>MSRVPSPPPPAEMSSGPVAESWCYTQIKVVKFSYMWTINNFSFCREEMGEVIKSSTFSSGANDKLKWCLRVNPKGLDEESKDYLSLYLLLVSCPKSEVRAKFKFSILNAKGEETKAMESQRAYRFVQGKDWGFKKFIRRDFLLDEANGLLPDDKLTLFCEVSVVQDSVNISGQNTMNMVKVPECRLADELGGLWENSRFTDCCLCVAGQEFQAHKAILAARSPVFSAMFEHEMEESKKNRVEINDVEPEVFKEMMCFIYTGKAPNLDKMADDLLAAADKYALERLKVMCEDALCSNLSVENAAEI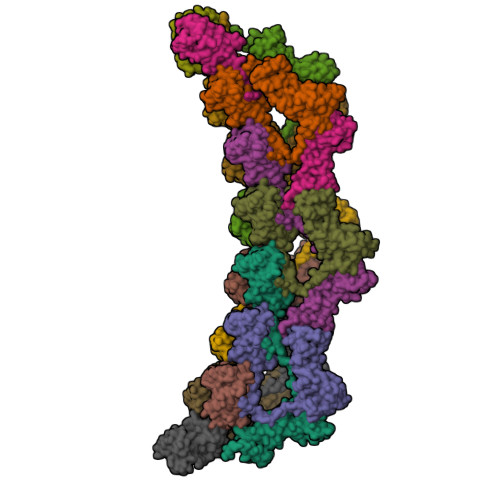LILADLHSADQLKTQAVDFINYHASDVLETSGWKSMVVSHPHLVAEAYRSLASAQCPFLGPPRKRLKQS[15x]MehpH is a monoalkyl phthalate hydrolases discovered from Gordonia sp. Strain P8219, a Gram-positive bacteria, and able to dissimilate several different kinds of monoester, such as MBP, MEP and MEHP18. Here we report the structures of MehpH, a monoalkyl phthalate (MBP) hydrolase that catalyzes the reaction of MBP to phthalic acid and the corresponding alcohol, in apo and ligand-bound form. The structure of MehpH, determined at a resolution of 2.3 Å, exhibits the typical fold of the α/β hydrolase superfamily and is composed of an α/β hydrolase core (residues 24-152 and 225-311) and an α-helical lid domain (residues 153-224). The tunnel is narrow in the body of the structure, but significantly enlarged at the substrate entrance, due to the flexibility of the NC-loop. The catalytic triad, composed of Ser125, Asp259 and His291 with His291 bridging Asp259 and Ser125 through hydrogen bonds, is situated at the bottle-neck of the tunnel, suggesting this tunnel may be involved in the hydrolysis process of MehpH.

The final construct used for crystallization contained a deletion of 23 amino acids on the N-terminus, which are predicted to be disordered. The twist β-sheet in the center of the α/β hydrolase core is formed by eight mixed β-strands (β1-β8) and surround by nine α-helices. Some residues in the the NC-loop (residues 153-164) that refers to a protein segment of variable length and structure linking β6 to the first structurally conserved helix in the lid domain were not assigned because of the discontinuity of the electron density. There is a penetrating tunnel formed by Loopβ3αA, αA, Loopβ5αD, Loopβ8αK and αK from the α/β hydrolase core and the NC-loop, αE, αF-αG from the lid domain. In the absence of MBP, the NC-loop becomes disordered to keep the the active site open. A Dali structural homology search revealed that MehpH shares the highest similarity with some meta-cleavage product hydrolases, with the Z-scores above 28.0 and root-mean-square deviation (RMSD) of 2.3–2.8 Å. Structure overlap exhibited that MehpH mainly shares high similarity with DxnB2 in the α/β hydrolase core, while their lid domains vary obviously, further supporting the ability of the α/β hydrolase core to accommodate different lid domains to achieve diverse substrate and chemical specificities.

>[2x]FHTVDVKGVQTRYFDDGQDKDPILLIHGGHFGFFIPVGIESWGNVLEDFGEYGRVLAVDKLGQGETGLPLNDEDWTVDAVAEHVANFATQLGLKNLTLVGHSRGGMTAVLLALKYPEMVKKLVIISSATAAPAPPVGTDMDFYERVERTAPGGSAELIRHYHAAQAVNEGDLPEDYIGIATKWLESEKQLDAVAGYARNAEEHWLPSLSEGRRWVQERLADAGIPVPTLVVWGVNDRSAPVSMGKGLFDLIAANTLDSSLYLINNAGHHVFSDQREKFNAAVGAFISL> MDVTCNIKNGRCEQFCKNSADNKVVCSCTEGYRLAENQKSCEPAVPFPCGRVSV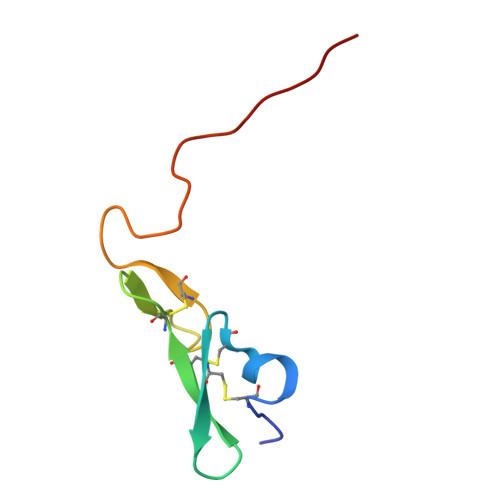SQTSKLTR>[2x]RSFIYEPFQIPSGSMMPTLLIGDFILVEKFAYGIKDPIYQKTLIETGHPKRGDIVVFKYPEDPKLDYIKRAVGLPGDKVTYDPVSKEL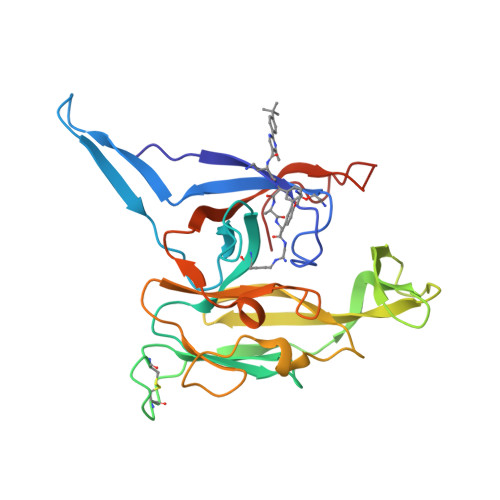TIQPGCSSGQACENALPVTYSNVEPSDFVQTFSRRNGGEATSGFFEVPKNETKENGIRLSERKETLGDVTHRILTVPIAQDQVGMYYQQPGQQLATWIVPPGQYFMMGDNRDNSADSRYWGFVPEANLVGRATAIWMSFDKQEGEWPTGLRLSRIGGIH> MSKAEKFYSLACYHAQLFSKDPNTKVAALVIDNNNNI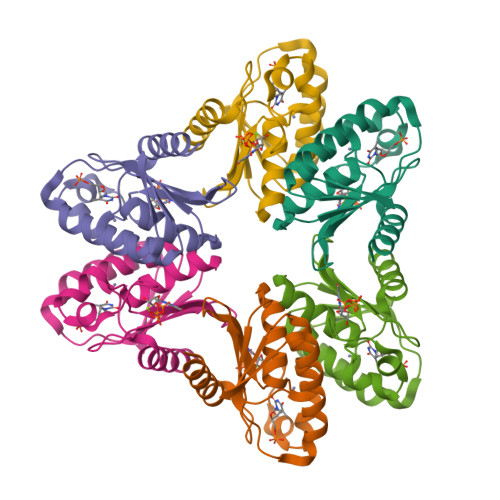ASVGYNGLPRGFEETSDRWEKPMKYNYVVHAQANAIATAARNGVRLDGCSIITTLFPCKECSKLIIQSGIRKVITSKPCKDSSWLESFSFSNEMFDECGIEVEYL Murrayamine-I | C20 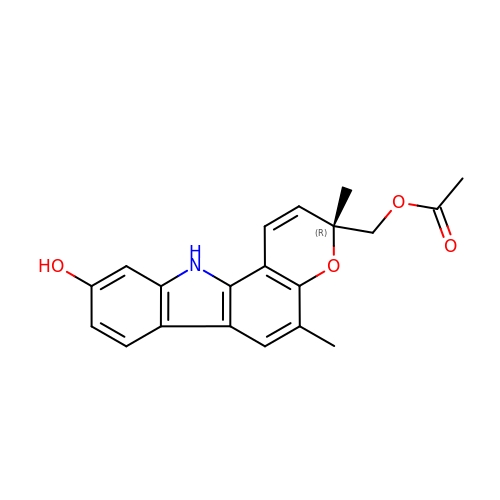H19 N O4 | HGIQTDGMLIBTAD-HXUWFJFHSA-N> MSKFLDRFRYFKQKGETFADGHGQLLNTNRDWEDGYRQRWQHDKIVRSTCGVNCTGSCSWKIYVKNGLVTWETQQTDYPRTRPDLPNHEPRGCPRGASYSWYLYSANRLKYPMMRKRLMKMWREAKALHSDPVEAWASII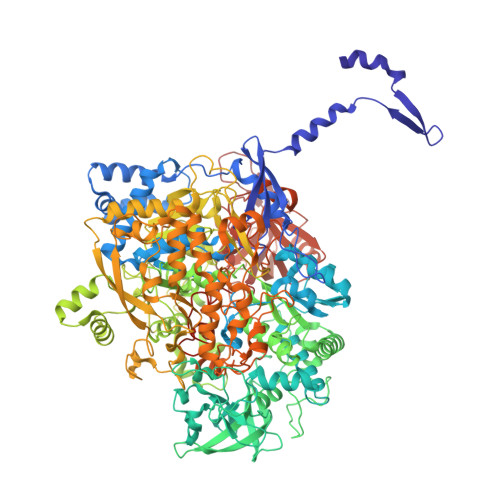EDADKAKSFKQARGRGGFVRSSWQEVNELIAASNVYTIKNYGPDRVAGFSPIPAMSMVSYASGARYLSLIGGTCLSFYDWYCDLPPASPQTWGEQTDVPESADWYNSSYIIAWGSNVPQTRTPDAHFFTEVRYKGTKTVAVTPDYAEIAKLCDLWLAPKQGTDAAMALAMGHVMLREFHLDNPSQYFTDYVRRYTDMPMLVMLEERDGYYAAGRMLRAADLVDALGQENNPEWKTVAFNTNGEMVAPNGSIGFRWGEKGKWNLEQRDGKTGEETELQLSLLGSQDEIAEVGFPYFGGDGTEHFNKVELENVLLHKLPVKRLQLADGSTALVTTVYDLTLANYGLERGLNDVNCATSYDDVKAYTPAWAEQITGVSRSQIIRIAREFADNADKTHGRSMIIVGAGLNHWYHLDMNYRGLINMLIFCGCVGQSGGGWAHYVGQEKLRPQTGWQPLAFALDWQRPARHMNSTSYFYNHSSQWRYETVTAEELLSPMADKSRYTGHLIDFNVRAERMGWLPSAPQLGTNPLTIAGEAEKAGMNPVDYTVKSLKEGSIRFAAEQPENGKNHPRNLFIWRSNLLGSSGKGHEFMLKYLLGTEHGIQGKDLGQQGGVKPEEVDWQDNGLEGKLDLVVTLDFRLSSTCLYSDIILPTATWYEKDDMNTSDMHPFIHPLSAAVDPAWEAKSDWEIYKAIAKKFSEVCVGHLGKETDIVTLPIQHDSAAELAQPLDVKDWKKGECDLIPGKTAPHIMVVERDYPATYERFTSIGPLMEKIGNGGKGIAWNTQSEMDLLRKLNYTKAEGPAKGQPMLNTAIDAAEMILTLAPETNGQVAVKAWAALSEFTGRDHTHLALNKEDEKIRFRDIQAQPRKIISSPTWSGLEDEHVSYNAGYTNVHELIPWRTLSGRQQLYQDHQWMRDFGESLLVYRPPIDTRSVKEVIGQKSNGNQEKALNFLTPHQKWGIHSTYSDNLLMLTLGRGGPVVWLSEADAKDLGIADNDWIEVFNSNGALTARAVVSQRVPAGMTMMYHAQERIVNLPGSEITQQRGGIHNSVTRITPKPTHMIGGYAHLAYGFNYYGTVGSNRDEFVVVRKMKNIDWLDGEGNDQVQESVK We provide an important correlation of a genome‐based mutation to a molecular phenotype across two predominant clinical Mtb lineages of the Indian subcontinent. We have identified a distinct lineage specific mutation‐G247C, translating into an alanine‐proline conversion in the papA2 gene of Indo‐oceanic lineage 1 (L1) Mtb strains, and restoration of cell wall sulfolipids by simple genetic complementation of papA2 from lineage 3 (L3) or from H37Rv (lineage 4‐L4) attributed the loss of this glycolipid to this specific mutation in Indo‐Oceanic L1 Mtb.

The investigation of structure of Mtb PapA2 revealed a distinct nonribosomal peptide synthetase (NRPS) C domain conformation with an unconventional presence of a zinc binding motif. Surprisingly, the A83P mutation did not map to either the catalytic center in the N‐terminal subdomain or any of the substrate‐binding region of the protein. On the contrary, the inherent ability of mutant PapA2 to form insoluble aggregates and molecular simulations with the wild‐type/mutant (Wt/mut) PapA2 purports an important role for the surface associated 83rd residue in protein conformation. This study demonstrates the importance of a critical structural residue in the papA2 protein of Mtb and helps establish a link between observed genomic alteration and its molecular consequence in the successful human pathogen Mtb.

>VFSITTLRDWTPDPGSIICWHASPTAKAKARQAPISEVPPSYQQAQHLRRYRDHVARGLDMSRLMIFTWDLPGRCNIRAMNYAINAHLRRHDTYHSWFEFDNAEHIVRHTIADPADIEVVQAEHQNMTSAELRHHIATPQPLQWDCFLFGIIQSDDHFTFYASIAHLCVDPMIVGVLFIEIHMMYSALVGGDPPIELPPAGRYDDHCVRQYADTAALTLDSARVRRWVEFAANNDGTLPHFPLPLGDLSVPHTGKLLTETLMDEQQGERFEAACVAAGARFSGGVFACAALAERELTNCETFDVVTTTDTRRTPTELRTTGWFTGLVPITVPVASGLFDSAARVAQISFDSGKDLATVPFDRVLELARPETGLRPPRPGNFVMSFLDASIAPLSTVANSDLNFRIYDEGRVSHQVSMWVNRYQHQTTVTVLFPDNPIASESVANYIAAMKSIYIRTADGTLATLKPGT[2x]>[2x]MHHHHHHNL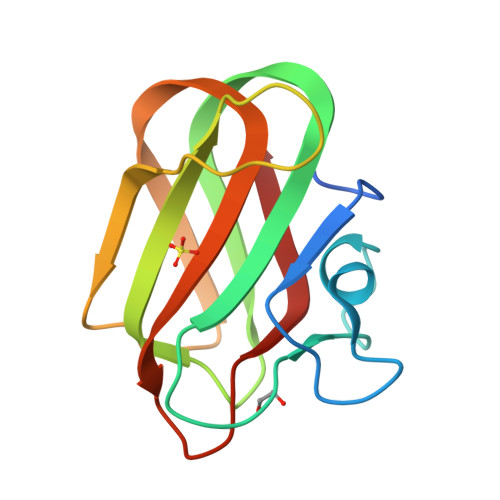ALNKATATSSIETAGHEGDKAVDGNAATRWASAYGASPQWIYINLGSTQSISRVKLNWEDAYATAYSIQVSNDSGSTPTNWTTVYSTTTGDGAIDDITFAATNAKFVRVYATTRATAYGYSLWEFEVYG> MSGQFTGTGTGGDVFKVDLNEQFD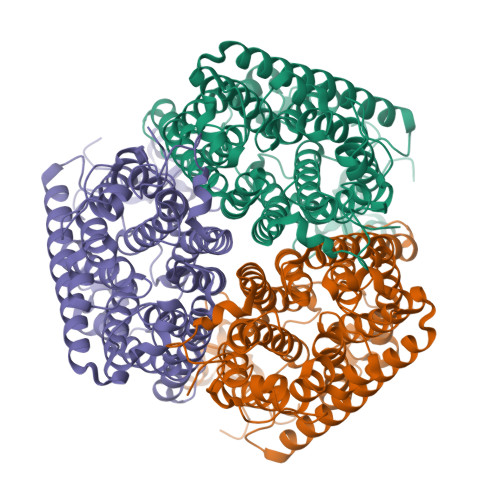RADMVWIGTASVLVWIMIPGVGLLYSGISRKKHALSLMWAALMAACVAAFQWFWWGYSLVFAHNGSVFLGTLQNFCLKDVLGAPSIVKTVPDILFCLYQGMFAAVTAILMAGAGCERARLGPMMVFLFIWLTVVYCPIAYWTWGGNGWLVSLGALDFAGGGPVHENSGFAALAYSLWLGKRHDPVAKGKVPKYKPHSVSSIVMGTIFLWFGWYGFNGGSTGNSSMRSWYACVNTNLAAATGGLTWMLVDWFRTGGKWSTVGLCMGAIAGLVGITPAAGYVPVYTSVIFGIVPAIICNFAVDLKDLLQIDDGMDVWALHCVGGFVGNFMTGLFAADYVAMIDGTEIDGGWMNHHWKQLGYQLAGSCAVAAWSFTVTSIILLAMDRIPFLRIRLHEDEEMLGTDLAQIGEYAYYADDDPETNPYVLEPIRSTTISQPLPHIDGVADGSSNNDSGEAKNHHHHHH>[2x]GSPGIRMSVETIIERIKARVGAVDPNGPRK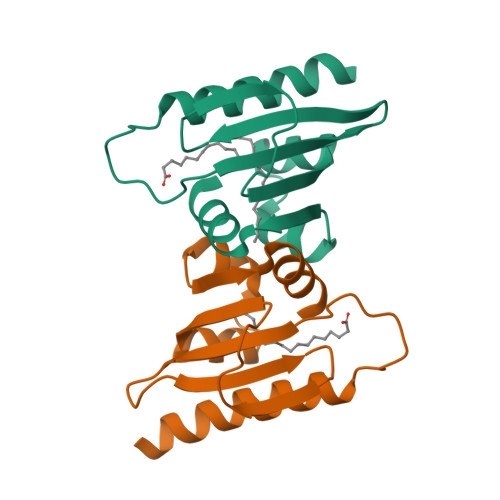VLGVFQLNIKTASGVEQWIVDLKQLKVDQGVFASPDVTVTVGLEDMLAISGKTLTVGDALKQGKIELSGDADLAAKLAEVI> SSADRLFPPQWICCDIRYLDVSILGKFAVVMADPPWDIHMELPYGTLTDDEMRRLNIPVLQDDGFLFLWVTGRAMELGRECLNLWGYERVDEIIWVKTNQLQRIIRTGRTGHWLNHGKEHCLVGVKGNPQGFNQGLDCDVIVAEVRSTSHKPDEIYGMIERLSPGTRKIELFGRPHNVQPNWITLGNQLDGIHLLDPDVVARFKQRYPDGIISKPKNL;> GSLKGTQSLNPHNDYCQHFVDTGHRPQNFIRDVGLADRFEEYPKLRELIRLKDELIAKSNTPPMYLQADIEAFDIRELTPKFDVILLEPPLEEYYRETGITANEKCWTWD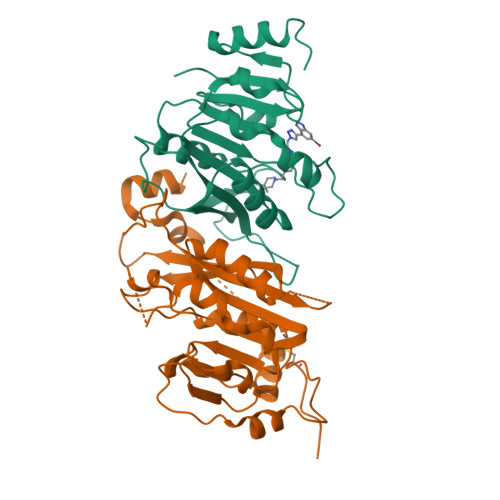DIMKLEIDEIAAPRSFIFLWCGSGEGLDLGRVCLRKWGYRRCEDICWIKTNKNNPGKTKTLDPKAVFQRTKEHCLMGIKGTVKRSTDGDFIHANVDIDLIITEEPEIGNIEKPVEIFHIIEHFCLGRRRLHLFGRDSTIRPGWLTVGPTLTNSNYNAETYASYFSAPNSYLTGCTEEIERL> MMENINIVIKDVGYFQDKPQFLNSKSVRQ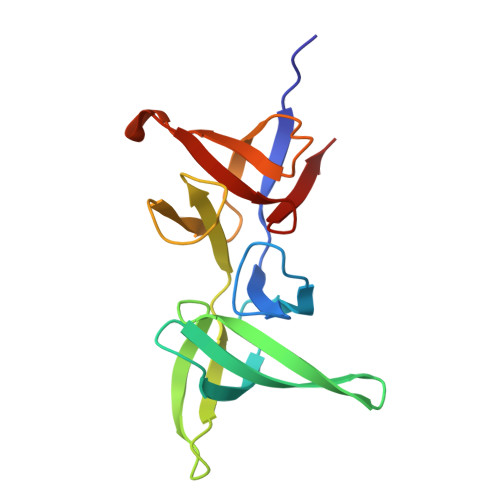WKHGTKVKLTKHNSHWYTGVVKDGNKSVRGYIYHSMAKVTSKNSDGSVNATINAHAFCWDNKKLNGGDFINLKRGFKGITHPASDGFYPLYFASRKKTFYIPRYMFDIKK> QCYHGNGQSYRGTFSTTVTGRTCQSWSSMTPHRHQRTPEN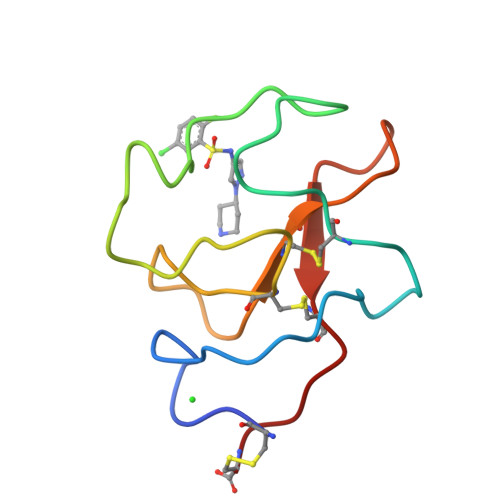YPNDGLTMNYCRNPDADTGPWCFTMDPSIRWEYCALTRC The Ton and Tol systems are sophisticated molecular machineries essential for virulence and survival of Gram-negative bacteria. Both systems rely on the proton gradient at the inner membrane to produce force and movement that are transmitted to target proteins associated with the outer membrane. Ton is involved in the uptake of essential nutrients such as siderophore-iron, vitamin B12 and carbohydrates, while Tol maintains outer membrane integrity and plays an active role in cell division. We have solved the high-resolution structures of the E. coli TonB-ExbB-ExbD and TolA-TolQ-TolR complexes, revealing the inner membrane embedded engine parts of the Ton and Tol systems, and showing how TonB and TolA interact with the ExbBD and TolQR subcomplexes.

To eventually detect structural heterogeneities and/or TonB binding at different ExbB, we performed an additional 3D classification step with the 227,384 particles that yielded the 2.8 Å resolution map. In these new orientations, TonB was found to bind ExbBE (18% of the particles) or ExbBA (13% of the particles). Except for the binding of TonB to different ExbB, the three structures do not show any noticeable structural difference for the ExbBD subcomplex, nor in the way TonB interacts with ExbB. As deduced from the TonB-ExbBD structures, one TonB subunit associates with ExbBD via ExbB chains C, E or A. The upper panel has the D-box bound to the ExbD periplasmic dimer in one orientation, leading to the binding of the TonB TM domain either to ExbBE (orange) or ExbBA (blue).

>[5x]MGNNLMQTDLSVWGMYQHADIVVKCVMIGLILASVVTWAIFFSKSVEFFNQKRRLKREQQLLAEARSLNQANDIAADFGSKSLSLHLLNEAQNELELSEGSDDNEGIKERTSFRLERRVAAVGRQMGRGNGYLATIGAISPFVGLFGTVWGIMNSFIGIAQTQTTNLAVVAPGIAEALLATAIGLVAAIPAVVIYNVFARQIGGFKAMLGDVAAQVLLLQSRDLDLEASAAAHPVRVAQKLRAG;> MTLDLPRRFPWPTLLSVCIHGAVVAGLLYTSVHQVIELPAPAQPISVTMVTPADLEPPQAVQPPPEPVVEPEPEPEPIPEPPKEAPVVIEKPKPKPKPKPKPVKKVQEQPKRDVKPVESRPASPFENTAPARLTSSTATAATSKPVTSVASGPRALSRNQPQYPARAQALRIEGQVKVKFDVTPDGRVDNVQILSAKPANMFEREVKNAMRRWRYEPGKPGSGIVVNILFKINGTTEIQGGGSENLYFQGGSAWSHPQFEK;>MAMHLNENLDDNGEMHDINVTPFIDVMLVLLIIFMVAAPLATVDVKVNLPASTSTPQPRPEKPVYLSVKADNSMFIGNDPVTDETMITALNALTEGKKDTTIFFRADKTVDYETLMKVMDTLHQAGYLKIGLVGEETAKAKENLYFQGNAGSGHHHHHHHHHH[2x]>GSHMRRLQQTQAQVDEVVDIMRVNVDKVLERDQKLSELDDRADALQAGASQFETSAAKLKRKYWWKNLKMMIILGVICAIILIIIIVYFST[2x];>GSHMDSSISKQALSEIETRHSEIIKLENSIRELHDMFMDMAMLVESQGEMIDRIEYNVEHAVDYVERAVSDTKKAVKYQSKARRKKIMIIICCVILGIIIASTIGGIFG[2x];>GSHMRNELEEMQRRADQLADESLESTRRMLQLVEESKDAGIRTLVMLDEQGEQLDRVEEGMNHINQDMKEAEKNL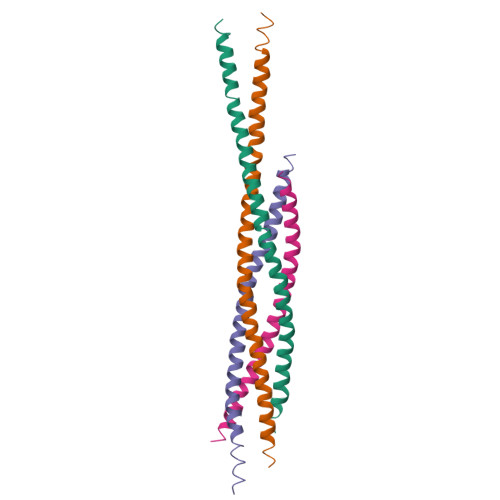KDLGK[2x];>GSHMARENEMDENLEQVSGIIGNLRHMALDMGNEIDTQNRQIDRIMEKADSNKTRIDEANQRATKMLG[2x]> GSHMEIYPHIKVYEGTLSRLKPGGAMIAVLEYDVNELSKHGYTNLWDVQFKVLVGVPHAETGVIYDPVYEETVKPYQPSNNLTGKKLYNVSTND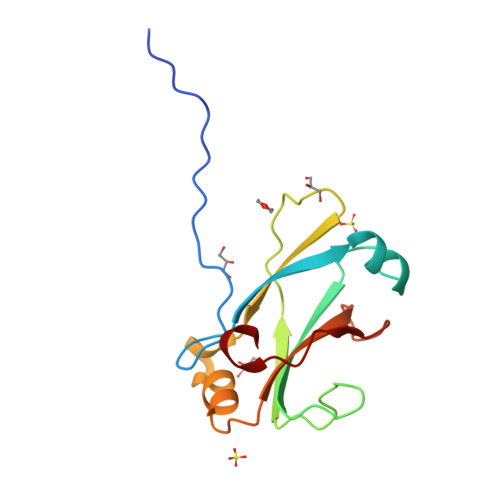MHNGYKWSNTMFSNSNYKTQILLTKGDGSGVKLYSKAYSENFK>[2x]MTTPSMEDYIEQIYMLIEEKGYARVSDIAE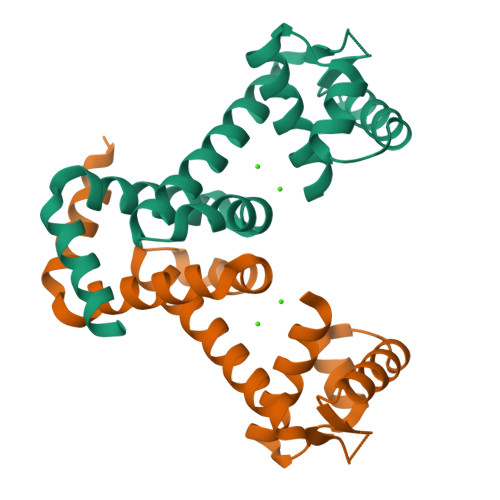ALAVHPSSVTKMVQKLDKDEYLIYEKYRGLVLTSKGKKIGKRLVYRHELLEQFLRIIGVDEEKIYNDVEGIEHHLSWNSIDRIGDLVQYFEEDDARKKDLKSIQKKTEHHNQ>SNAYSIALIIPSLFEKACAHFLPSFQQALNKAGYQLLLGYSDYSIEQEEKLLSTFLESRPAGVVLFGSEHSQRTHQLLEASNTPVLEIAELSSKASYLNIGVDHFEVGKACTRHLIEQGFKNVGFIGARGNHSTLQRQLHGWQSAMIENYLTPDHFLTTHEAPSSQLGAEGLA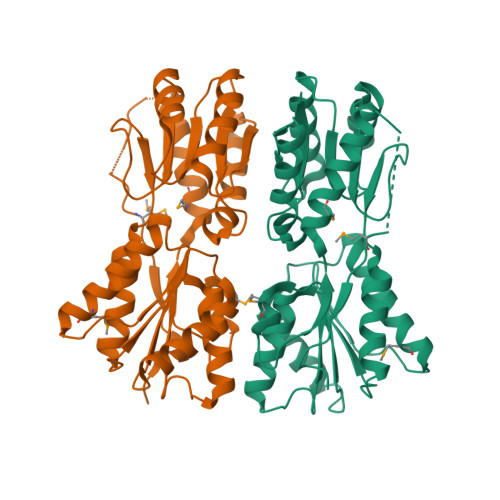KLLLRDSSLNALVCSHEEIAIGALFECHRRVLKVPTDIAIICLEGSSMGEHAYPSLTSAEFDYERMGTKAAEKLLHAIKGEPEERPTSMGFKLKRRASTAIN[2x]> GFPTELKPGTNQFLTTDDGTSPPILPGFEPTPLIHIPGEFTSLLDLCQIETILEVNNTTSTTGVSRLLIPVRAQNNVDQLCASFQVDPGRNGPWQSTMVGQICRYYTQWSGSLKVTFMFTGSFMATGKMLIAYTPPG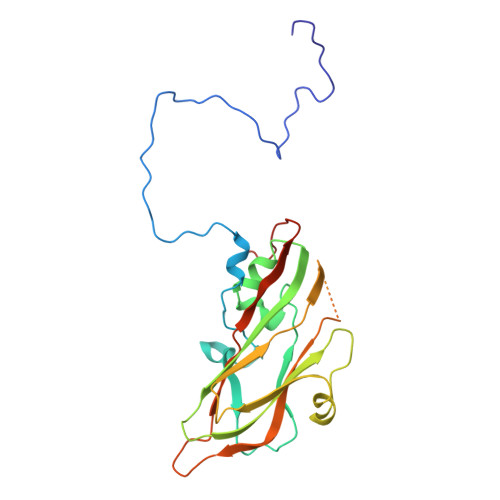SAQPATREAAMLGTHIVWDFGLQSSVTLVIPWISNTHFRAVKTGGVYDYYATGIVTIWYQTNFVVPPDTPTEANIIALGAAQKNFTLKLCKDTDEIQQTAEYQ>MKSVVTTVIAAADAAGRFPSSSDLESVQGSIQRSAARLEAAEKLGANLDNVAQEAYNACIQKYPYLNNAGEANSNDTYKAKCLRDVKHYMRLI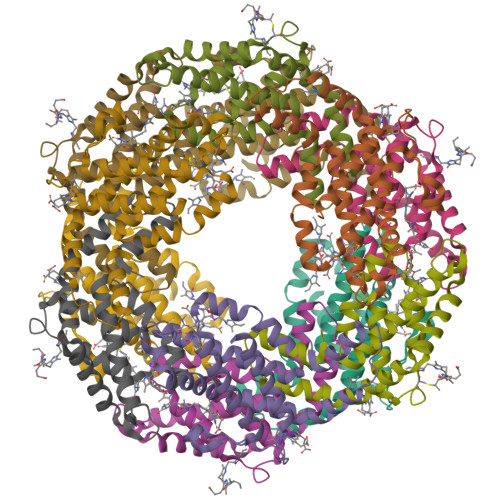QYCLVVGGTGPLDEWGIAGQREVYRALSLPTAPYVEALSFARNRGCAPRDMSAQALVEYNALLDYAINSLS[12x];>MLDAFSRAVVQADASTSVVGDVSALKQFIAQGNRRLDAVNAIASNASCMVSDAIAGMICENQGLIQAGGNCYPNRRMAACLRDGEIILRYVTYALLAGDASVLDDRCLNGLKETYAALGVPTTSTVRAVQIMKAQAAAHIKDTPSEARAGAKLRKMGSPVVEDRCSSLVAEASSYFDRVIAALS[12x]> VENSGAGPTSFKTMKVIDPQHSDKPNVLILGSGWGAISFLKHIDTKKYNVSIISPRSYFLFTPLLPSAPVGTVDEKSIIEPIVNFALKKKGNVTYYEAEATSINPDRNTVTIKSLSAVSQLYQPENHLGLHQAEPAEIKYDYLISAVGAEPNTFGIPGVTDYGHFLKEIPNSLEIRRTFAANLEKANLLPKGDPERRRLLSIVVVGGGPTGVEAAGELQDYVHQDLRKFLPALAEEVQIHLVEALPIVLNMFEKKLSSYAQSHLENTSIKVHLRTAVAKVEEKQLLAKTKHEDGKITEETIPYGTLIWATGNKARPVITDLFKKIPEQNSSKRGLAVNDFLQVKGSNNIFAIGDNAFAGLPPTAQVAHQEAEYLAKNFDKMAQIPNFQKNLSSRKDKIDLLFEENNFKPFKYNDLGALAYLGSERAIATIRSGKRTFYTGGGLMTFYLWRILYLSMILSARSRLKVFFDWIKLAFFKRDFFKGL

A monotopic alternative NADH dehydrogenase (Type II NADH dehydrogenase: NDH-2) catalyses the electron transfer from NADH to quinone via FAD or FMN without a proton-pumping activity, and functions as an initial enzyme, either in addition to or as an alternative to proton-pumping NADH dehydrogenase (complex I) in the respiratory chain of bacteria, archaea, and fungal and plant mitochondria. A series of studies has suggested that Ndi1, one of three NDH-2s from Saccharomyces cerevisiae, would be useful in replacement therapy for mitochondrial diseases caused by complex I dysfunction. We reported that the enzymatic reaction of yeast Ndi1 has a ping-pong mechanism, as is the case with NDH-2s from Mycobacterium tuberculosis and Yarrowia lipolytica. In this reaction mechanism, two substrates—NADH and ubiquinone—bind to the enzyme sequentially, but not at the same time.

A Lineweaver-Burk plot analyses indicated that stigmatellin is a competitive inhibitor whereas the others are mixed-type. The crystal of Ndi1-stigmatellin contains one Ndi1 and two bound stigmatellin molecules in the asymmetric unit. Two stigmatellin molecules, STG-1 and STG-2 are bound to the hydrophobic surface of the membrane-anchor region of Ndi1. STG-1 is located at the si-face of the adjacent FAD cofactor in the cavity formed by the C-terminal α15 helix and the β19-21 sheets of Ndi1. The aromatic head groups of the STG-1a and STG-1b overlap each other, while the aliphatic tails extend to different directions. The aromatic head groups of the STG-1a and STG-1b form hydrogen bonds with the isoalloxazine ring of the FAD cofactor and are surrounded by W63, P92, A393, Q394, H397, A446, L447, Y482, M485, and L487 (site 1 in Figs 4A and 5). In contrast, STG-2 is bound to a groove formed by helixes α15 and α16 in the C terminal membrane-anchor domain of Ndi1. In contrast, STG-1a apparently overlaps with the previously reported ubiquinone binding site, UQI, while STG-1b overlaps with UQII.>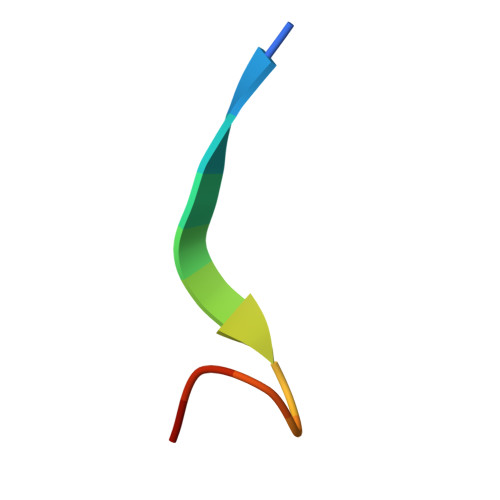 DDNTLYHRGFTED>[2x]GPYLVIVEQPKQRGFRFRYGCEGPSHGGLPGASSEKGRKTYPTVKICNYEGPAKIEVDLVTHSDPPRAHAHSLVGKQCSELGICAVSVGPKDMTAQFNNLGVLHVTKKNMMGTMIQKLQRQRLRSRPQGLTEAEQRELEQEAKELKKVMDLSIVRLRFSAFLRSLPLKPVISQP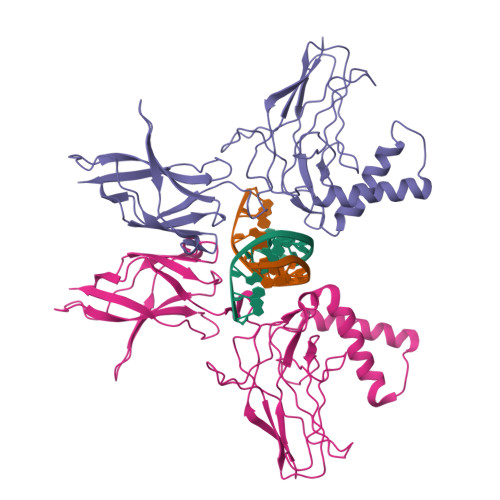IHDSKSPGASNLKISRMDKTAGSVRGGDEVYLLCDKVQKDDIEVRFYEDDENGWQAFGDFSPTDVHKQYAIVFRTPPYHKMKIERPVTVFLQLKRKRGGDVSDSKQFTYYP> MGDRVEELDTRETSLLVAEVKGWLMKLASGKGEISPSAYDTAWVARIPSESDSSLPEFPEALEWIINSQLPDGSWGDDRHLQLYDRVLSTLSCLVTLKTWDIGHNSIAQGTKFLRENMIKLKQDDGDLLSGFEVTFPMMLHEAKQLGLDIPYETEFTRLLEISTKKKLAKIPLDKIHSAPTTLLYSLEGLQDLEIDWQKILKLQSKDGSFLSSPSSTACVYLKTKGRKSLQYLQNAMEDQNYAVPCHYPIDLFESLWVVDTIERLGIDVFFRDEIKAVLDYVYSFWTNEGIGWGSTCLVNDIDDTAMAFRILRMHGYNVSTDAFNQFWLPGDKFCCFVGELSHGVSEMLNLHRASQVDFPNEAILTKTFKYSHDYLLNVDSAHMDKWATKKNLMGEVAFELANPFHDCLPRIYNNAYIKHYGMDDLWIAKTIYRLPLVNNKVFLELANRYAQQCQLYQPAELTKLVNWWHSSRFEDIPSTRLTANIDMLPYIYYVICATFHEQEFAQLRVFFSKACCLNTLFDDLMDCATSIEELDRLQNVIEKWDISLSHELPLEYRIPFQEFYNTVLVMTEAASKIHKNLSPEFICKYLSGIYTKLIKSEIADARWKIEGYIPSFEEYMENAEVSISTWVHVLMSILFCGEPLTEEILNTIYDSRPLKLDRIICRLCNDIQTYKIEMKLGQPTQGVSCYMKEHPGATEEDALVYLQSLLEKTKRELNESYFITHENDLPKN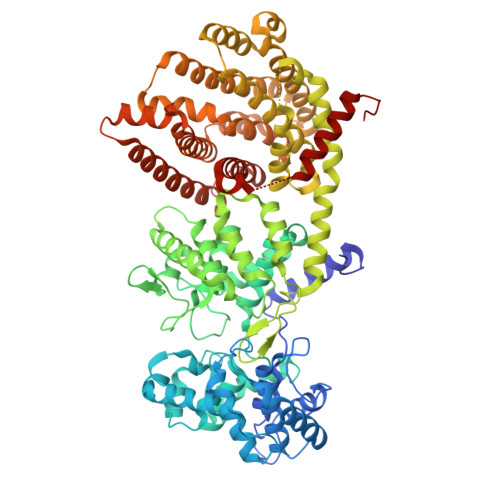IKRFNFEMVRMMLITYNETRQVDLFRNPDNELKDMIKFCLETYRTLLEHHHHHH>[2x]GSHMMNDGKQQSTFLFHDYETFGTHPALDRPAQFAAIRTDSEFNVIGEPEVFYCKPADDYLPQPGAVLITGITPQEARAKGENEAAFAARIHSLFTVPKTCILGYNNVRFDDEVTRNIFYRNFYDPYAWSWQHDNSRWDLLDVMRACYALRPEGINWPENDDGLPSFRLEHLTKANGIEHSNAHDAMADVYATIAMAKLVKT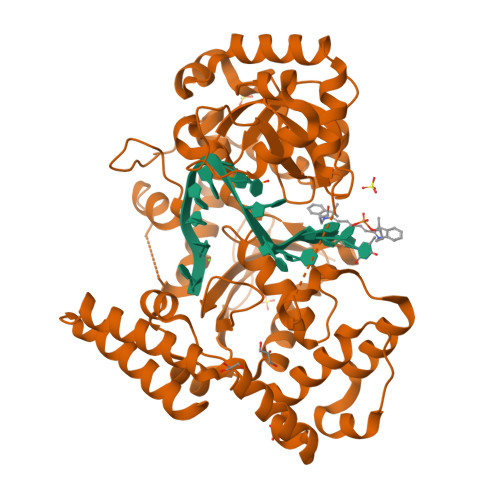RQPRLFDYLFTHRNKHKLMALIDVPQMKPLVHVSGMFGAWRGNTSWVAPLAWHPENRNAVIMVDLAGDISPLLELDSDTLRERLYTAKTDLGDNAAVPVKLVHINKCPVLAQANTLRPEDADRLGINRQHCLDNLKILRENPQVREKVVAIFAEAEPFTPSDNVDAQLYNGFFSDADRAAMKIVLETEPRNLPALDITFVDKRIEKLLFNYRARNFPGTLDYAEQQRWLEHRRQVFTPEFLQGYADELQMLVQQYADDKEKVALLKALWQYAEEIV> HHHHHSSGVPRGSHMRILVIAGCSEGFVMPLVPLSWALRAAGHEVLVAASENMGPTVTGAGLPFAPTCPSLDMPEVLSWDREGNRTTMPREEKPLLEHIGRGYGRLVLRMRDEALALAERWKPDLVLTETYSLTGPLVAATLGIPWIEQSIRLASPELIKSAGV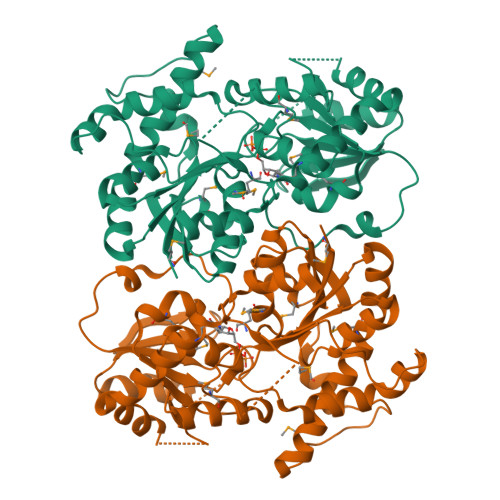GELAPELAELGLTDFPDPLLSIDVCPPSMEAQPKPGTTKMRYVPYNGRNDQVPSWVFEERKQPRLCLTFGTRVPLPNTNTIPGGLSLLQALSQELPKLGFEVVVAVSDKLAQTLQPLPEGVLAAGQFPLSAIMPACDVVVHHGGHGTTLTCLSEGVPQVSVPVIAEVWDSARLLHAAGAGVEVPWEQAGVESVLAACARIRDDSSYVGNARRLAAEMATLPTPADIVRLIEQA Mammalian lipocalin and secretoglobin allergens are associated with a function in chemical communication that involves abundant secretion into the environment, high stability and the ability to transport small volatile compounds. Lipocalins are a highly diverse protein family and on average, its members (allergens and non-allergens) share <30% amino acid sequence identity. They all feature highly conserved β-barrel structures that enable them to transport small volatile hydrophobic compounds. Guinea pig allergen Cav p 1 isoallergens are found in hair and are expressed in the harderian gland. Furthermore, we solved the crystal structure of the major guinea pig allergen Cav p 1, a lipocalin closely related to the well-known semiochemical hamster aphrodisin, allowing us to compare the binding cavities of mammalian respiratory allergens belonging to three different lipocalin subgroups.

We could solve the crystallographic structure of Cav p 1.0101 at 3.7 Å. The crystal belongs to the P212121 space group with five molecules in the asymmetric unit. Cav p 1.0101 adopts a classic lipocalin fold: an eight stranded β-barrel (residues 9-112) with a short helix insertion between β1 and β2, followed by a 14 residue long α-helix and a short β-strand forming antiparallel interactions with β1. The crystal used to obtain the structure of Cav p 1.0101 was obtained in the presence of 1-decanol. An electron density that is observed in the central cavity of monomer E, likely indicates the presence of a 1-decanol molecule. In the four other monomers, the corresponding density is significantly weaker. This density is adjacent to the carbonyl oxygen of Ser14, one of the very few polar atoms on the surface of the cavity available for hydrogen bonding, which is likely involved in an H-bond with the hydroxyl group of 1-decanol. The Cav p 1.0101 cavity does not display any access to the solvent. The β-barrel side open to the solvent in the LCN1 structure is occupied by the sidechain of Phe74, which belongs to the short β5β6 loop in Cav p 1.0101. This loop, which is part of the interface between monomers in the crystal likely acts as a lid capable of opening for the ligands to access the central cavity. Based on our model protein Cav p 1.0101 we observed that the cavity inside the β-barrel is defined by the side chains of 17 mostly hydrophobic residues.

>[5x]MAEINGDWNTIALSADNKEKIEEGGPLRVYFRQVDCNDDCSEITFRLYVKLSGECKESTVIASQTPDDFYTVQFAGENTFLIVDKQEDLFTLYNTNVDENGLVTRGYAIIGKRDSLTPEETSHFEEANELKGIPKGNIEYLAGTDDCPERSHHHHHH> GAGCAGACCTG;> ACGCCACTCA;> CACGT;>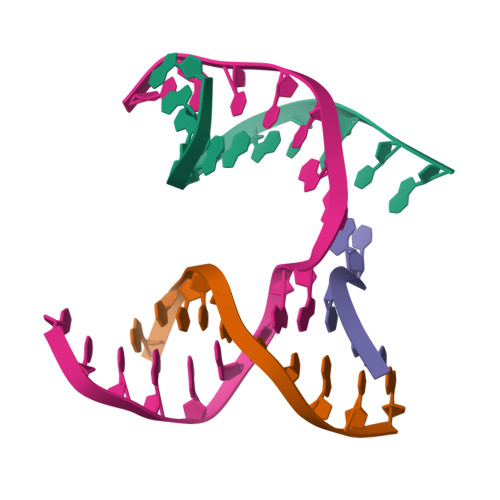 TCTGAGTGGGGTCTGC>GEVEYLCDYKKIREQEYYLVK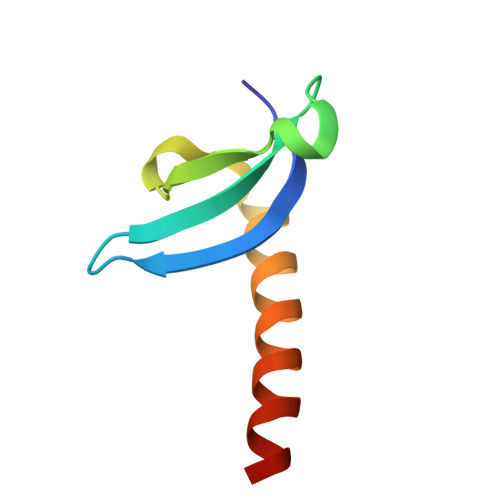WRGYPDSESTWEPRQNLKCVRILKQFHKDLERELLRRHHRSKT[3x]>GCGAGCCUAGCGAAGUCAUAAGCUAGGGCAGUCUUUAGAGGCUGACGGCAGGAAAAAAGCCUACGUCUUCGGAUAUGGCUGAGUAUCCUUGAAAGUGCCACAGUGACGAAGUCUCACUAGAAAUGGUGAGAGU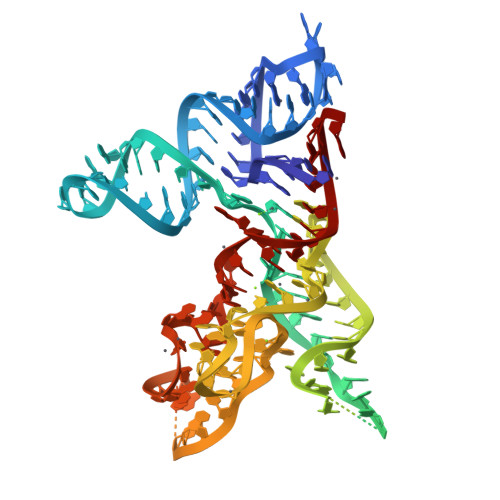GGAACGCGGUAAACCCCUCGCA[2x]> GPAMNSVFSGLDMLILLPYERRGTRLVVEDYRPDHIYCIGADFGKNQDYSVFSVL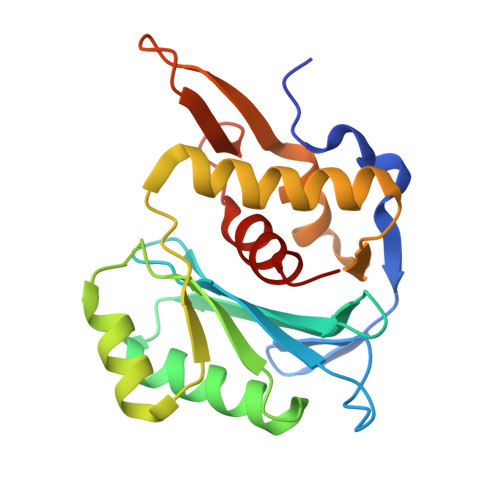DLDTGAIACLERMNGATWSDQVARLKALSEDYGHAYVVADTWGVGDAIAEELDAQGINYTPLPVKSSSVKEQLISNLALLMEKGQVAVPNDKTILDELRNFRYYRTASGNQVMRAYGRGHDDIVMSLALAYSQYEG> MGRDPNSSSVDKLAAALEHHHHHHMSAVASHVVPPRSKLDSILSSGLEHNIDHDPLEVWDKGVFLNELLKQGIALSTNENGTLDGELVADEGLKKGSYKGTRLALTEIYSILEDAAVSHFDKRGYEPIFPVKRELDLKKRIYQWSDGTDGYPPHLKVDGNDEANLPADERQSKPGSARSEGVGQIFDMQETAFVSKIAQAVSFIIPKDIDHENTPYKGPTLADVEKFNKAQFPKTDGDASNQDNLNKAADIMKGRNIGEYDDWYSDARFAQQHFSGVNPSTIETASQDKIK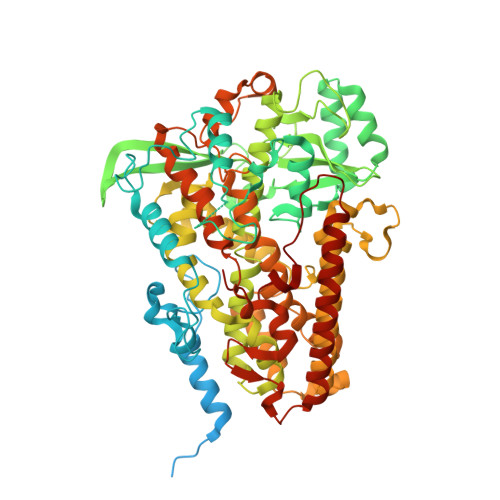EYISEAQKQGLDKVKAILEDGKDILIQDYSYFREATGATNEQIFQNTVYELKGTTPTGKTTSRYAAASVVIFQLHEDGRLHPLAITLDYKGSLDNSITIFNRRLSPDDTCDIAEKEDWPWRYAKTVAQTADWARHEVATHLVDTHMIEEAIIVATNRIIPEGELLYEILSPHWFRTLSLNAAARKLLVPGVIARIAGFGPTSPSLDFKGNNAFKLIDWSYKNFNFQDKYIPNDLKKRGFDIKGDKSGKYKNYPYANDMYLLWGIIRNFVKTVIESQYTSDHVVQKDPYIGGWCKEIQTNGQIPTFPTITTVEQLIDAVTMCIHTASPQHTAVNYLQDYYYSFVPAKPPALCTPLPQDLSALQGYTEKDLTAALPIGTEDMKWKDWLLAAQLPELLSYKVQQDYNLITYAKSLYNVNKNRTITENTKFNCKTIKKAAADFYSHLKSAGVEFENYSKGQTAGTVEYPVLQPETTAISILI> MLRKDIGIDLGTANTLVFLRGKGIVVNEPSVIAIDST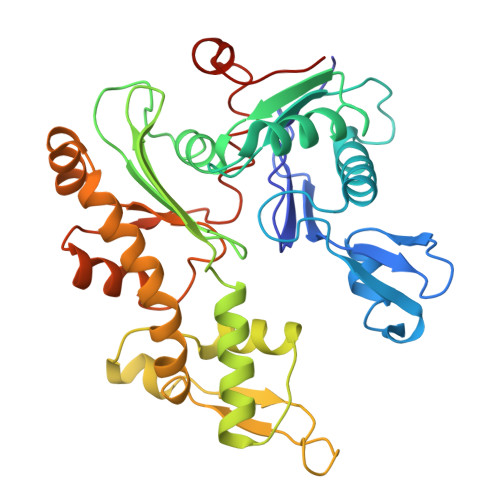TGEILKVGLEAKNMIGKTPATIKAIRPMRDGVIADYTVALVMLRYFINKAKGGMNLFKPRVVIGVPIGITDVERRAILDAGLEAGASKVFLIEEPMAAAIGSNLNVEEPSGNMVVDIGGGTTEVAVISLGSIVTWESIRIAGDEMDEAIVQYVRETYRVAIGERTAERVKIEIGNVFPSKENDELETTVSGIDLSTGLPRKLTLKGGEVREALRSVVVAIVESVRTTLEKTPPELVSDIIERGIFLTGGGSLLRGLDTLLQKETGISVIRSEEPLTAVAKGAGMVLDKVNILKKLQGAGGSHHHHHH> AASVTAEKAALDITKMTPIHDRVLIRPIEEEQKTAGGILLPKAPPKANSDAHIGEVLAVGSDVTLAVAKGDMVVFQKYAMAE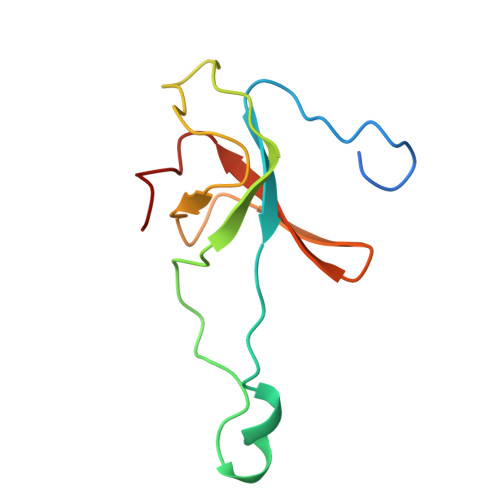VEVKEGQIIFVAEKSIMGKLE Muramidases are N-acetylmuramide glycanhydrolases which cleave the β-1,4-glycosidic bond between N-acetylmuramic acid (NAM) and N-acetylglucosamine (NAG) in the carbohydrate backbone of the bacterial cell-wall peptidoglycan. Here, the identification, characterization and X-ray structure of a novel fungal GH24 muramidase from Trichophaea saccata is first described, in which an SH3-like cell-wall-binding domain (CWBD) was identified by structure comparison in addition to its catalytic domain. A ‘domain-walking’ approach, searching for other sequences with a domain of unknown function appended to the CWBD, was then used to identify a group of fungal muramidases that also contain homologous SH3-like cell-wall-binding modules, the catalytic domains of which define a new GH family. The properties of some representative members of this family are described as well as X-ray structures of the independent catalytic and SH3-like domains of the Kionochaeta sp., Thermothielavioides terrestris and Penicillium virgatum enzymes.

Attempts were made to crystallize the full-length enzymes from T. terrestris and P. virgatum. However, in both cases the enzyme was cleaved at the much longer (than in the GH24 family) linker between the domains. The crystals of the T. terrestris enzyme contained only the catalytic GH184 domain, which was closely similar to that from Kionochaeta sp. The P. virgatum crystal, in contrast, only contained the SH3-like CWBD, which was similar in fold to the GH24 CWBD. The full-length protein consists of an N-terminal CWBD followed by a catalytic domain. However, the CWBD was lost during crystallization, so the structure starts from Gly85 and only contains the catalytic domain. The fold is closely similar to that of KsGH184, with the largest differences in the loop region close to the active-site entrance: the r.m.s.d. is 1.8 Å for 204–213 equivalent Cα positions in TtGH184 (excluding residue 208), corresponding to residues 120–129 in Kionochaeta versus 0.75 Å for the full-length catalytic domains (superposed by SSM as incorporated in Coot; Krissinel & Henrick, 2004). There are two zinc ions from the crystallization medium, one coordinated by His132 (corresponding to the cadmium-coordinating His63 in KsGH184), Glu135 and two waters, and the other coordinated by His170 from three symmetry-related molecules and possibly water, or some unidentified compound from crystallization/protein production. Glu125 in TtGH184 corresponds to the catalytic Glu41 in KsGH184 (Glu45 in gp13), and Asp150 in TtGH184 (Asp66 in KsGH184) corresponds to Gln54 in gp13 that potentially stabilizes the ligand. The proposed flexibility of the linker explains the difficulty in obtaining crystals of the full-length protein and its apparent cleavage during crystallization experiments.

> YPVKADTLNCRSGPGTSYKVIKTYKKGTDLKITCQTPGTSVNGDNLWDKTSDGCYVADYYVKTGTSGYVTAHCDAGSGSGSSGGGNLPGLNSVQSSHARAIIGEAKKEGVGRHGCEAGIATALVESNILIYANKAVPASLKYPHDAVGSDHDSVGIFQQRAKYYPNIAADMDPARSAAQFFAKMKGIKGWQSMAVGTLCQKVQGSAYPDRYAKRVSEATKICQAGGL> ACCC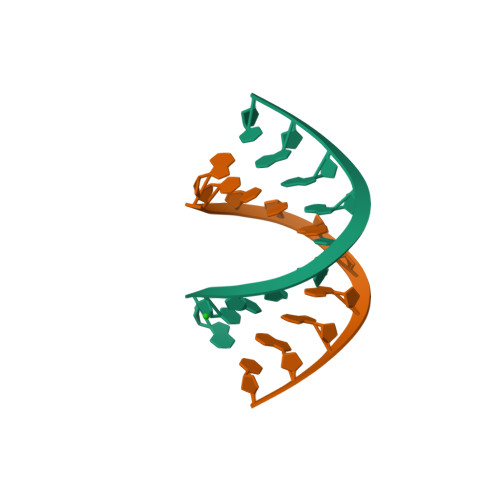GCGGGT> MVREAGEVVAIVPAAGSGERLAVGVPKAFYQLDGQTLIERAVDGLLDSGVVDTVVVAVPADRTDEARQILGHRAMIVAGGSNRTDTVNLALTVLSGTAEPEFVLVHDAARALTPPALVARVVEALRDGYAA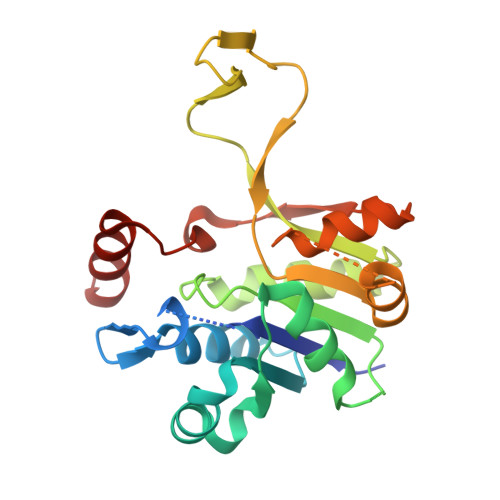VVPVLPLSDTIKAVDANGVVLGTPERAGLRAVQTPQGFTTDLLLRSYQRGSLDLPAAEYTDDASLVEHIGGQVQVVDGDPLAFKITTKLDLLLAQAIVRG> GGUCAUGAGUGCCAGCGUCAAGCCCCGGCUUGCUGGCCGGCAACCCUCCAACCGCGGUGGGGUGCCCCGGGUGAU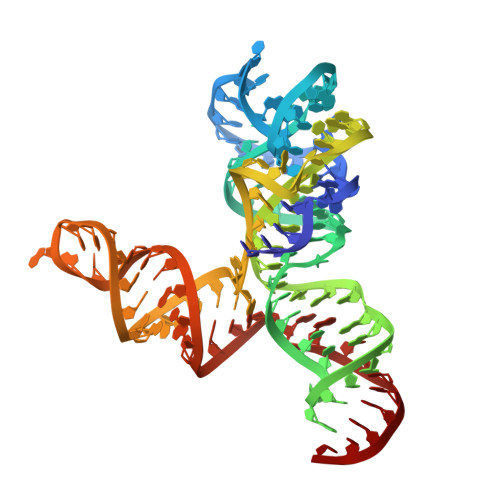GACCAGGUUGAGUAGCCGUGACGGCUACGCGGCAAGCGCGGGUC> MASMTGGQQMGRDLQVTLYGTIKAGVEVSRVKDAGTYKAQGGKSKTATQIADFGSKIGFKGQEDLGNGMKAIWQLEQKASIAGTNSGWGNRQSFIGLKGGFGTVRAGNLNTVLKDSKDNVNAWESGSNTEDVLGLGTIGRVESREISVRYDSPVFAGFSGSVQYVPRDNANDVDKYKHTKSSRESYHAGLKYENAGFFGQYAGSFAKYADLN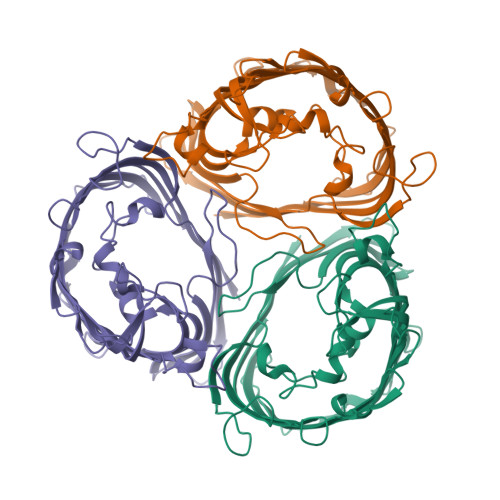TDAERVAVNTANAHPVKDYQVHRVVAGYDANDLYVSVAGQYEAAKNNEVGSIKGKKHEQTQVAATAAYRFGNVTPRVSYAHGFKAKVNGVKDANYQYDQVIVGADYDFSKRTSALVSAGWLKQGKGAGKVEQTASMVGLRHKF> PGRPRLAPPQNVTLLSQNFSVYLTWLPGLGNPQDVTYFVAYQSSPTRRRWREVEECAGTKELLCSMMCLKKQDLYNKFKGRVRTVSPSSKSPWVESEYLDYLFEVEPAPPVLVLTQTEEILSANATYQLP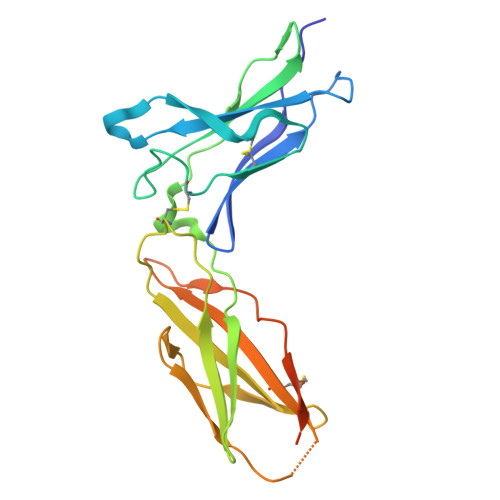PCMPPLDLKYEVAFWKEGAGNKTLFPVTPHGQPVQITLQPAASEHHCLSARTIYTFSVPKYSKFSKPTCFLLEVPEANASGSSGGSSGTSHHHHHH> MGSSHHHHHHSSGRENLYFQGMNISEINGFEVTGFVVRTTNADEMNPMTA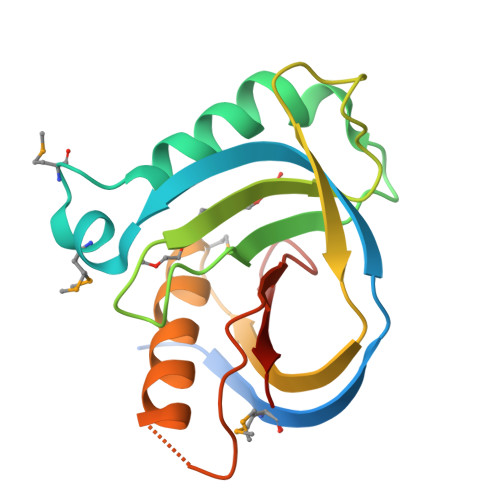KIGNLWEKFYLNAAPKLTDKSKVYGLYTNYESDFTGAFDVIACSDTLSPQLLSESVKTKVSSGKYVTFSATGEMPQVVIDLWNEVWNYFASEHCPHKRAYTTDFEYYKSANTVEISIAVR> MLGPKRCSMVLDVAFVLEGSDKIGEADFNRSKEFMEEVIQRMDVGQDSIHVTVLQYSYMVTVEYPFSEAQSKGDILQRVR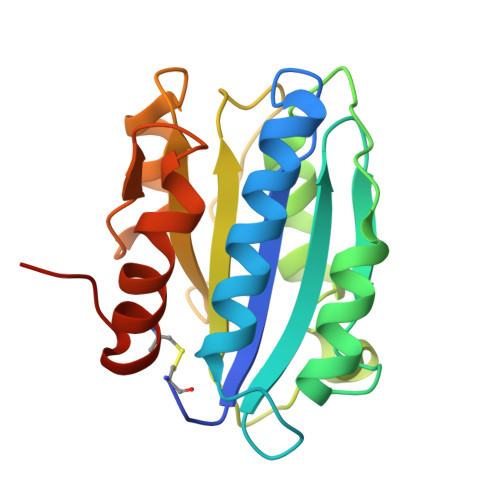EIRYQGGNRTNTGLALRYLSDHSFLVSQGAREQAPNLVYMVTGNPASDEIKRLPGDIQVVPIGVGPNANVQELERIGWPNAPILIQDFETLPREAPDLVLQRCSSGEGLEHHHHHH> SIERLGYLGFAVKDVPAWDHFLTKSVGLMAAGSAGDAALYRADQRAWRIAVQPGELDDLAYAGLEVDDAAALERMADKLRQAGVAFTRGDEALMQQRKVMGLLCLQDPFGLPLEIYYGPAEIFHEPFLPSAPVSG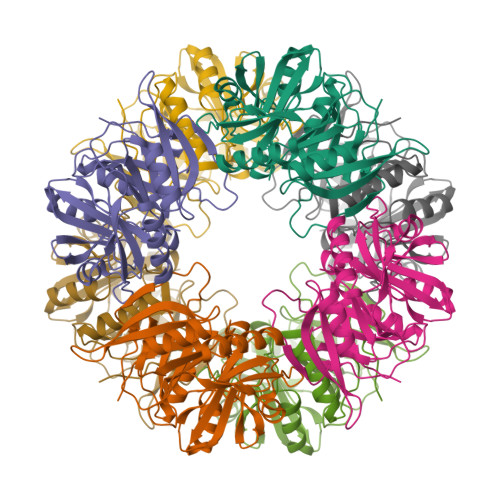FVTGDQGIGHFVRCVPDTAKAMAFYTEVLGFVLSDIIDIQMGPETSVPAHFLHCNGRHHTIALAAFPIPKRIHHFMLQANTIDDVGYAFDRLDAAGRITSLLGRHTNDQTLSFYADTPSPMIEVEFGWGPRTVDSSWTVARHSRTAMWGHKSVRGQR> GPHMRTISYSEARQNLSATMMKAVEDHAPILITRQNGEACVLMSL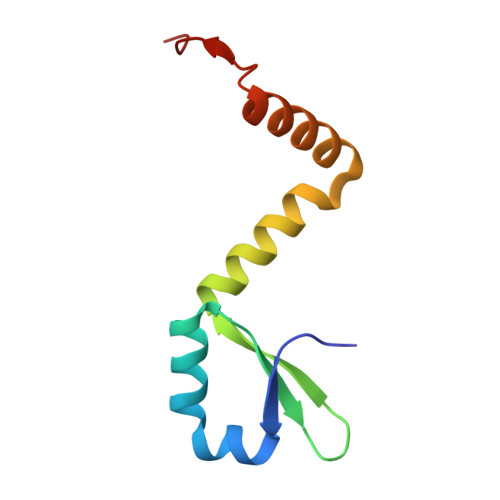EEYNSLEETAYLLRSPANARRLMDSIDSLKSGKGTEKDIIE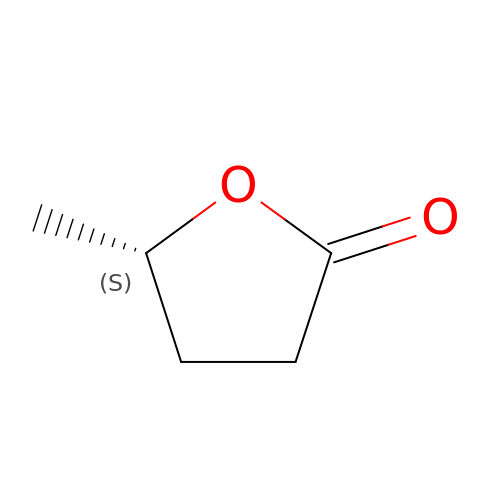gamma-Valerolactone | C5 H8 O2 | GAEKPEKOJKCEMS-BYPYZUCNSA-N>MTIQDFQSSGKATVLAVGTAVPPKEFDQSTYPDFYFNVTNCNDKVELKGKFQRICDRSGIKKRHFYLDEEILKANPGMCTYMGASLDVRQNIAVREVPKLAKEAALKAIKEWGQPKSKITHLVFGTTSGVDMPGADFQLLKLLGLRPNVKRIMLYQQGCSAGATVT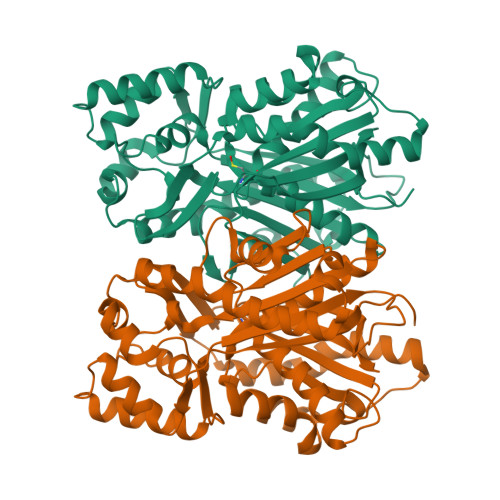RVAKDLAENNPGARVLVACSEVTAVTFRAPSETHLDGLVGAALFGDGAAALIIGSNPTPVEKPLFEVHWSGQCVLPDSDGAILGHLREAGLVFHLLKDVPGIISKNIEKLLAEPLDYVKSVDEASPAYTDLFWVVHPGGPAILDQVEAKLKLDKDRMQATRDVLAQYGNMSSASVLFVLDQMRKRSVELNKDTTGDGLKWGVMLGFGPGLTVETLLLKSI[2x]Ca2+/calmodulin-dependent protein kinase II (CaMKII) is a Ser/Thr kinase that is particularly important in neuronal signaling and cardiac function. CaMKII has a unique architecture, in which the catalytic domains are linked flexibly to a hub domain, also called the association domain, which forms a dodecameric or tetradecameric assembly (see Figure 1A for a description of the domains of CaMKII). We reported recently that the activation of CaMKII-α by ATP and Ca2+/CaM triggers the exchange of activated subunits between different holoenzyme assemblies. Our data are consistent with the idea that the CaM-binding element induces the hub to transition from a closed-ring form to a ring-opened lock-washer configuration, which can release or capture dimer units.

The hub domain of CaMKII-A crystallized at pH 7, while that of CaMKII-B crystallized at pH 4.2. The N-terminal α helix of the CaMKII-B hub is preceded by a 12-residue segment of the variable linker, including several acidic residues. In the structure of the N. vectensis CaMKII-B hub at pH 4.2, this segment is ordered in every subunit, and it folds back to dock onto the central β-sheet of the same hub subunit, extending the β-sheet by one strand, as seen in the structure described earlier for human CaMKII-α. The acidic sidechains in this segment are located close to the acidic residues in the hub. This particular configuration is unexpected, and is presumably possible only because some or all of the acidic residues are protonated at the low pH of crystallization. Comparison of the N. vectensis CaMKII-B hub at pH 4.2 with that of tetradecameric or dodecameric hubs shows that the linker peptide cannot be accommodated within the grooves of the closed-ring forms without steric clashes. The assembly is distorted at each interface in a systematic way throughout. This leads to the formation of a spiral, similar to a “lock-washer”, with a slight opening between the A-B and M-N dimers (subunit notation is indicated in Figure 6D). The segment that is bound at the interfacial grooves in the ruptured N. vectensis structure is not the CaM-binding element, which was not part of the crystallization construct. Instead it is the C-terminal portion of the linker, which is presumably accommodated due to the low pH of crystallization.

>GPHTIIEEDTESTKTQREQEIIRLTQQLITSITAKDFDSYSKLVDPKITAFEPEALGNQVEGLEFHKFYFDNLPNKRNTTVNTTILAPHVQMLGEEGACISYVRLTQGIGPDGLPRTTQSEETRVWQKKKGVWLNVHFHRSVSRP[7x]> SHMEDQLSRR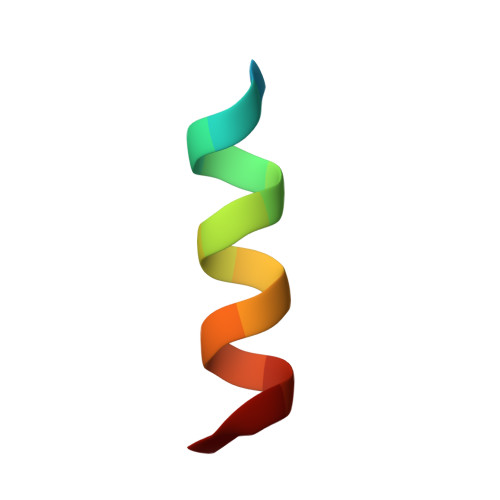LAALRN N-{(2S)-1-({(2S)-1-[(2,4-difluorobenzyl)amino]-1-oxopropan-2-yl}amino)-4-[(2S)-2-methylpiperidin-1-yl]-1,4-dioxobutan-2-yl}-5-methyl-1,2-oxazole-3-carboxamide (non-preferred name) 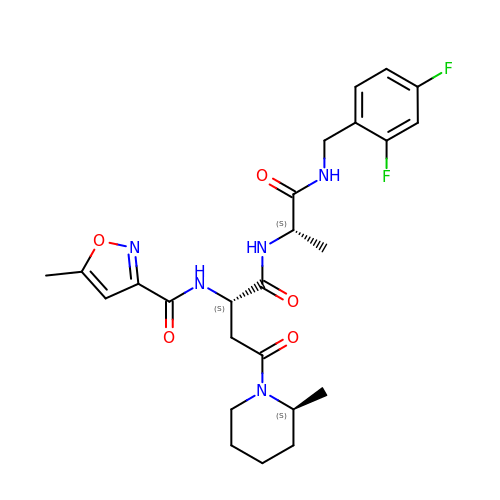| C25 H31 F2 N5 O5 | XOTJQAONWIKZEB-UVFQYZLESA-N> MRKWQC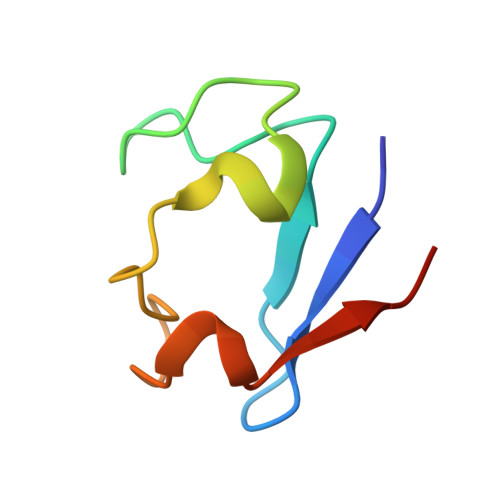VVCGFIYDEALGLPEEGIPAGTRWEDIPADWVCPDCGVGKIDFEMIEIA Droxinostat | C11 H14 Cl N O3 | 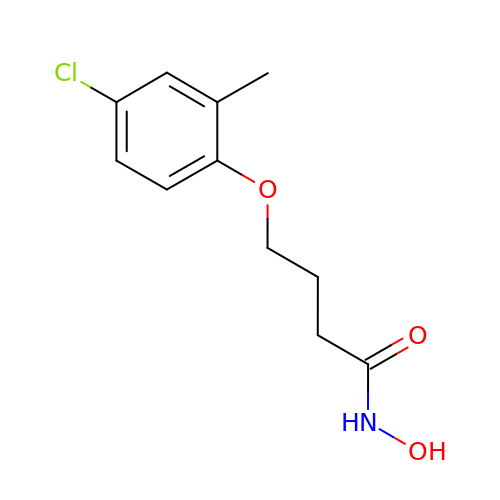JHSXDAWGLCZYSM-UHFFFAOYSA-N>MTSVEDLYVVKPINQWPAPSGLPVPSPPGTLLPGQSPDEAFARNSVVFLVPGAEYNWKNVVIRKPVWIYGNGATVKTSGLGPIIHIMGDLDNPMDVRIQDLTFIGGDSPDRLVPFSAVLTNQMALWCIDPRITIRGCSFYNFGGAAIYLERSERDTGFRFGRGQVMITDCRFRGCRIGIANGGSVEYGLASQNNFSDCQICFNVVGGNWTRSGNVASNCRCMYLHTQGMWYEGAAGNFNPAHGSFTSNTLNHCDYGGNLWPTEFQLPDRVINLAGFYFDNAAARLPNFSGNSQWYGDMKLINFLPDSTFVINGGALYGGPGDTGVIAVATALAAKVFVI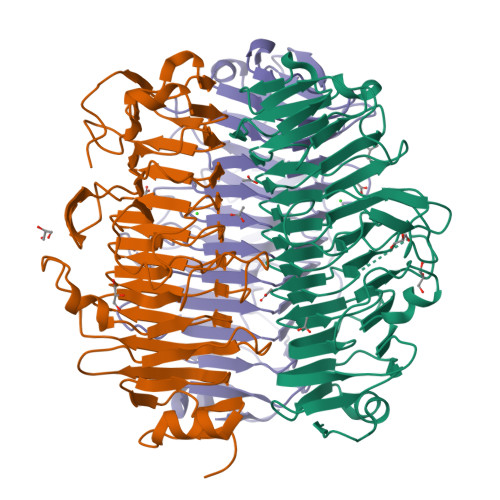GCQGNAGQQIVNVPAANIIPEVGTRKDDATQPAA[6x]4-{4-[(1H-benzimidazol-2-ylmethyl)amino]-6-(2-chloro-4-methoxyphenoxy)pyrimidin-2-yl}piperazin-2-one | C23 H22 Cl N7 O3 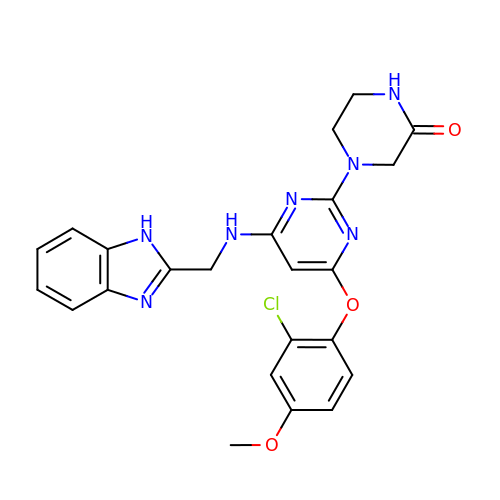| CWWLCYZCSRQXMN-UHFFFAOYSA-N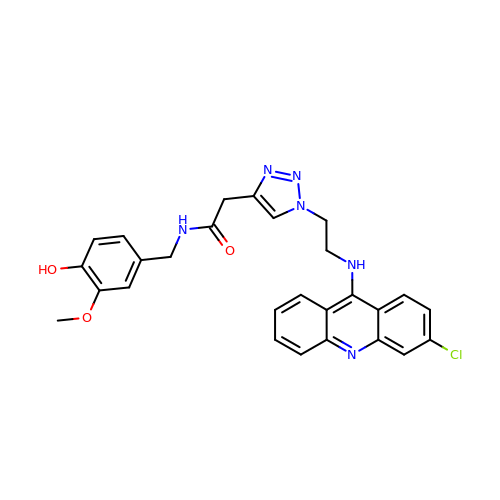2-[1-[2-[(3-chloranylacridin-9-yl)amino]ethyl]-1,2,3-triazol-4-yl]-~{N}-[(3-methoxy-4-oxidanyl-phenyl)methyl]ethanamide | C27 H25 Cl N6 O3 | UQMOCUNKULLJES-UHFFFAOYSA-N>GPGSSHWTSKVHESVIGRNPEGQLGFELKGGAENGQFPYLGEVKPGKVAYESGSKLV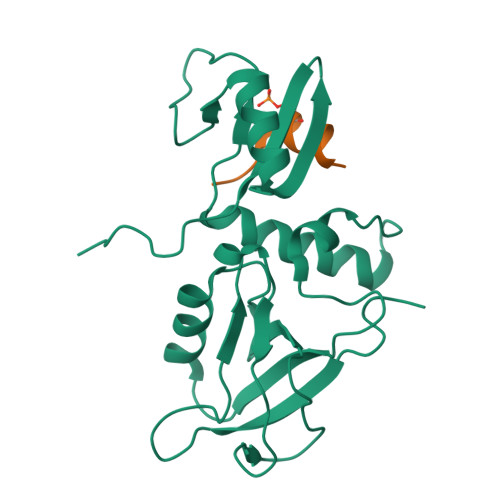SEELLLEVNETPVAGLTIRDVLAVIKHCKDPLRLKCVKQGGIVDKDLRHYLNLRFQKGSVDHELQQIIRDNLYLRTVPCTTRPHKEGEVPGVDYIFITVEEFMELEKSGALLESGTYEDNYYGTPKPPAEPAPLLNVTDQILPGATPSAEGKRKRNKSVTNMEKASIEPPEEEEEER[2x];>[2x]GLRSTSYRRAVV The Fc IgG binding protein (FCGBP), found in intestinal mucus secretions and other extracellular environments, contains 13 VWD domains, 11 of which have a GDPH cleavage site. Many VWD domains have a glycine‐aspartate‐proline‐histidine (GDPH) amino‐acid sequence motif, which is hydrolytically cleaved post‐translationally between the aspartate (Asp) and proline (Pro). FCGBP has been reported to bind the Fc portion of antibodies (Harada et al., 1997) and factors involved in innate immunity (Houben et al., 2019), and it has been suggested to help clear mucosal surfaces of trapped pathogens (Kobayashi et al., 2021). In this study, we used a representative FCGBP D assembly to determine how GDPH cleavage affects VWD stability and structure, as well as to explore the chemical mechanism of cleavage.

Based on these initial findings, a truncated variant containing only the VWD and C8 domains, spanning amino acid residues 4073–4349, was prepared. This variant crystallized in the same space group (P212121) with similar unit cell dimensions (43.72 × 54.32 × 129.11 Å) as the longer version (44.94 × 54.23 × 126.75 Å) but provided improved diffraction data, to 2.2 Å resolution. In FCGBP D10, the C8 domain was not packed against the side of the VWD β‐sandwich but instead was perched atop the sandwich, interacting with an S‐shaped loop that in turn packs against the extended hairpin between β‐strands β5 and β6. One notable feature of the cleaved motif is that the peptide bond before the aspartate (the Gly‐Asp bond) is unambiguously in the cis configuration. The cis peptide enables the Asp to make backbone hydrogen bonds to both the hairpin with which C8 interacts and, via a water molecule, to the loop between β‐strands β13 and β14 in the fold. Another notable feature of the cleavage site in the D10 structure is that the backbone carboxylate carbon of the aspartate and the proline nitrogen are 6.3 Å apart, as opposed to about 1.3 Å in a peptide bond. In this orientation, the Asp side chain is in position to hydrogen bond with the side chain of the GDPH His. In cleaved FCGBP D10, this loop forms a β‐hairpin that leans over the β‐sheet containing the GDPH motif. One of the β‐strands of the hairpin is in position to form a backbone hydrogen bond from a carbonyl to the N‐H group of the aspartate in the GDPH motif, as well as to the new N‐H group of proline generated upon peptide cleavage. We found that endogenous Asp‐Pro cleavage increases the resistance of the domain to exogenous proteolytic degradation.

> APATCWLWGD;> PHYHSFDGRKFDFQGTCNYVLATTGCPGVSTQGLTPFTVTTKNQNRGNPAVSYVRVVTVAALGTNISIHKDEIGKVRVNGVLTALPVSVADGRISVAQGASKALLVADFGLQVSYDWNWRVDVTLPSSYHGAVCGLCGNMDRNPNNDQVFPNGTLAPSIPIWGGSWRAPGWDPLCWDECRGSCPTCPEDRLEQYEGPGFCGPLASGTGGPFTTCHAHVPPESFFKGCVLDVCMGGGDHDILCKTLASYVAACQAAGVVIEDWRAQVGCEHHHHHH>[2x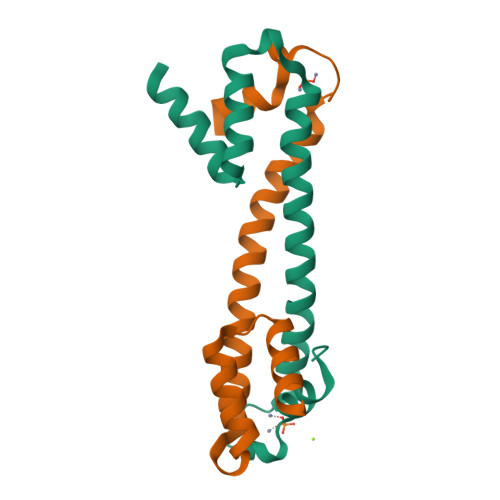]SDLQRLKFIRHARQLGFSLESIRELLSIRIDPEHHTCQESKGIVQERLQEVEARIAELQSMQRSLQRLNDACCGTAHSSVYCSILEALEQGASGVKSGC> VSLDPARTDRPYLLGRLFAVLEKAQEDAVPGANATIKDRYLASASANPGQVFHMLLKNASNHTAKLRKDPE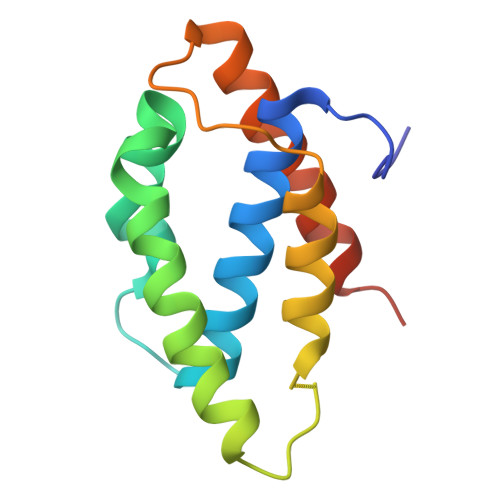RKGSAIHYEIMMQEIIDNISDFPVTMSSDEQGLFMIGYYHQRKALFTKKNKEN>[2x]MAELTALHTLTAQMKREGIRRLLVLSGEEGWCFEHTLKLRDALPGDWLWISPRPDAENHCSPSALQTLLGREFRHAVFDARHGFDAAAFAALSGTLKAGSWLVLLLPVWEEWENQPDADSLRWSDCPDPIATPHFVQHLKRVLTADNEAILWRQNQ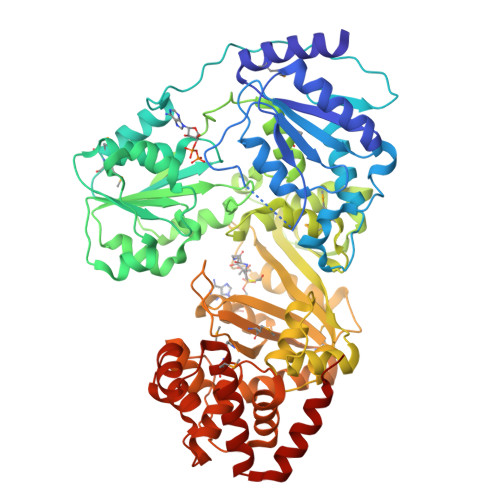PFSLAHFTPRTDWYPATGAPQPEQQQLLKQLMTMPPGVAAVTAARGRGKSALAGQLISRIAGRAIVTAPAKASTDVLAQFAGEKFRFIAPDALLASDEQADWLVVDEAAAIPAPLLHQLVSRFPRTLLTTTVQGYEGTGRGFLLKFCARFPHLHRFELQQPIRWAQGCPLEKMVSEALVFDDENFTHTPQGNIVISAFEQTLWQSDPETPLKVYQLLSGAHYRTSPLDLRRMMDAPGQHFLQAAGENEIAGALWLVDEGGLSQQLSQAVWAGFRRPRGNLVAQSLAAHGNNPLAATLRGRRVSRIAVHPARQREGTGRQLIAGALQYTQDLDYLSVSFGYTGELWRFWQRCGFVLVRMGNHREASSGCYTAMALLPMSDAGKQLAEREHYRLRRDAQALAQWNGETLPVDPLNDAVLSDDDWLELAGFAFAHRPLLTSLGCLLRLLQTSELALPALRGRLQKNASDAQLCTTLKLSGRKMLLVRQREEAAQALFALNDVRTERLRDRITQWQLFH> MPNLFDPLRVGDLNLPNRVVMAPLTRLRAGPTHIPNALMAEYYGQRASAGLLITEGVPVAPQGVGYAGVPGIWSKEQTEGWKQVTKAVHDKGGRIFMQIWHVGRISDPELLNGELPIAPSAIAAKGHVSLLRPQRDYPTPRALSTEEVAGVVEAFRQGAENAQAAGF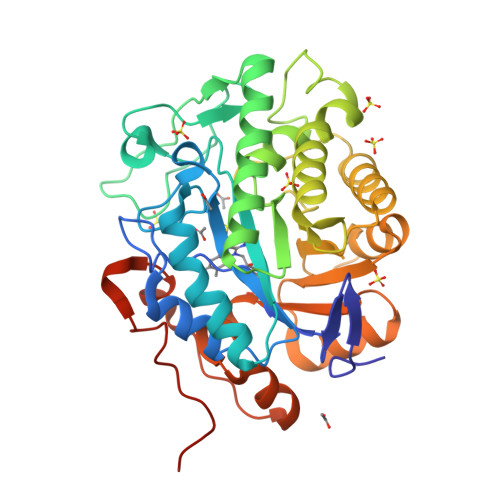DGVQLHGANGYLLDQFLQDGSNQRTDQYGGSIENRARLLLEAADAAISVWGADRVGVHLAPRADSHSMGDSNLAATFGHVAKALGERKIGFVSAREYEAADSLGPDLKKAFGGVYIANEKFDLASANAAIEAGKADAIAFGKAYIANPDLVERLKAGAALNTPDPATFYGFENGPRGYTDYPTLAQVREPALEHHHHHH> MARAYSLLSSRNRLIPRVEVQCRKREWVKTDPDSPFLNGGREVLY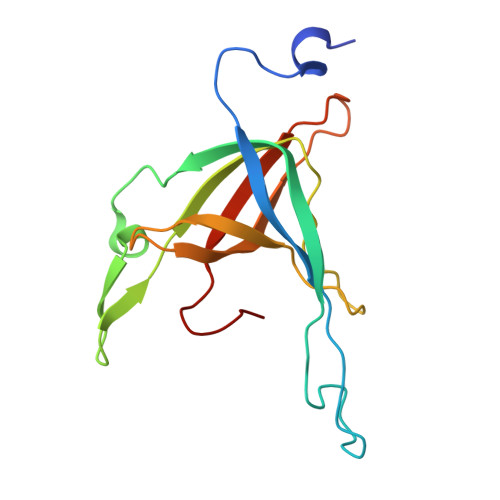TPFTAVECTVQPMRGKAIRDQNNQLMIGGEEDYDSYTVYSETLLFRAREGTEHLSDQMLLPDSGGGQTWFTVMKADMYPSSGVPRYRYYLIAVPVGTEGGL> MSSVFDEYEQLL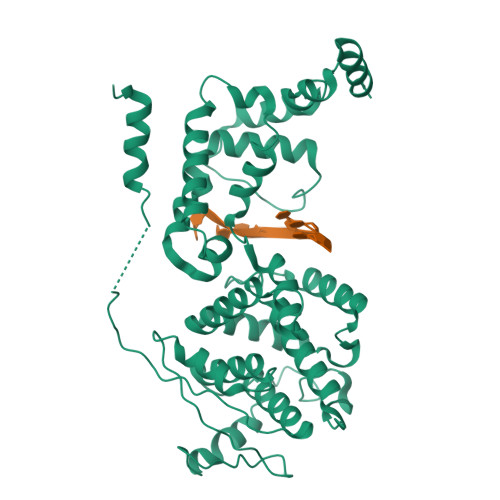AAQTRPNGALGGGEKGSTLKVEVPVFTLNSDDPEDRWNFAVFCLRIAVSEDANKPLRQGALISLLCSHSQVMRNHVALAGKQNEATLAVLEIDGFTNGVPQFNNRSGVSEERAQRFMMIAGSLPRACSNGTPFVTAGVEDDAPEDITDTLERILSIQAQVWVTVAKAMTAYETADESETRRINKYMQQGRVQKKYILHPVCRSAIQLTIRQSLAVRIFLVSELKRGRNTAGGTSTYYNLVGDVDSYIRNTGLTAFFLTLKYGINTKTSALALSSLSGDIQKMKQLMRLYRMKGDNAPYMTLLGDSDQMSFAPAEYAQLYSFAMGMASVLDKGTGKYQFARDFMSTSFWRLGVEYAQAQGSSINEDMAAELKLTPAARRGLAAAAQR>GHMRTNKDRLVRISVVGEIAPAKMRSPYSVTTEGTVRVIPVLGGITYNVK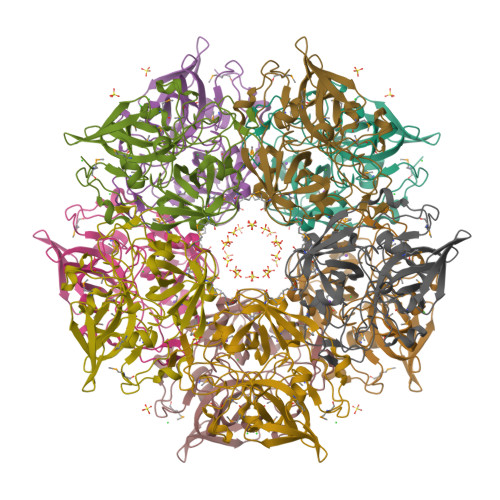VGDSAYGWAGDHVEPGVSVMARRKEEEIPLMTLSCIGNEVIVMSGDAKGSRGFVTGKHGGVNHVLVHFEEEVLGKLMVGDKILIKAWGQGLKLLDHPDVKVMNIDPDLFEKLGIQEKNGKIHVPVVAKIPAHMMGSGIGASSSASTDYDIMASNPEDLGVADLKLGDIVAIQDHDNSYGVGKYRKGAVSIGVVVHSACVSAGHGPGVVVIMTGDESKILPEEVERANISDYLVR[5x]>[2x]MNMTKYIPVLQSLLFVLLLSFSGHAQEHPSLILTKAGVEKIRAELGNIPIFDATLEKVKAEVDAEIALGIDTPLPKDYSGGYTHERHKRNFFILQKAGVLYQILNDEKYALYIKDMLFQYEGMYKDLPVHPQTRSYARGKLFWQCLNDS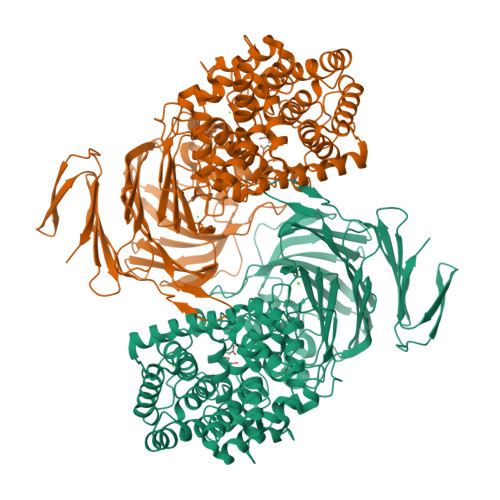NWLVYVSQAYDCVYDYLSKKERKQLEKNLFRPFADYISIENPQFYNRVHNHSTWGNAAVGMIGLVMGDEELIQRALYGIEDDGLPIGAKDNDGGFIKVEGQKAGFLANIDEPFSPDGYYTEGPYYQRYAMYPFLIFAEALHNVRPQQKIFEHKDGVLLKSVNTLLSLSDADGEFFPLNDAQKGMSYHSRELVTAVDIAYHYGNHNPQLLSIAEEQGQVLLDDSGLAVALGIREGKSEDFQKKSIKLSDGANGDQGGVAILRYGNEAMTLVYKYAAQGLSHGHYDKLSFSLYEKGTEILQDYGLARFVNIEQKGGGNYLKENTTWAKQTIAHNTLVQNETSHFEGKYEVGSQHHSELYFFDASNPEVQVVSAKEQNAYPGTEMHRTMALIKTDGFEKPFVLDILRVGSNAANQYDLPFYFKGQVMQTNFDFTTPKSLEPLGSDNGYQHLWSEGLGQPKGDNSQLSWLENGRFYTLTTATNNDDELHFVRIGANDPEFNLRRDAGLIIRRKNTKNTTFVSILESHGHYSPVSEFSVNANSSISKIELMLDTKEYTAVLIDAKSNTEQTLLILANENKNVNKEHIIEIKGKEYRWTGPYQFIKIN> MSLPKPEDVLVAPNFGIQIDGVMVEYLNSVSNLQIEQDVIRYQQNQGTTGRNNVTLMPGVAKDGSVQVERGMSQSSVFTQWINDSMAGRMATARKNATIIVMDYEDNPVKRWNLR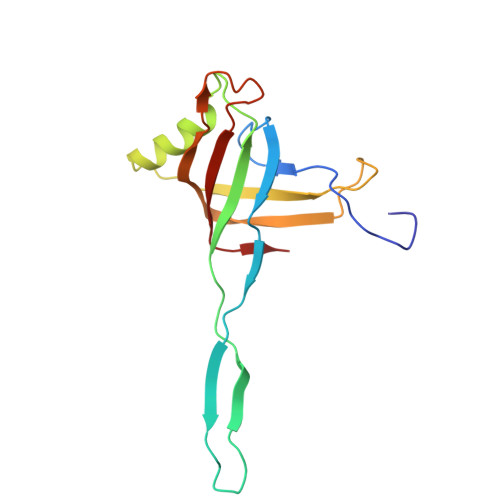NAWCSKVVAGTLKAGDTNALTETITIVFEELVVE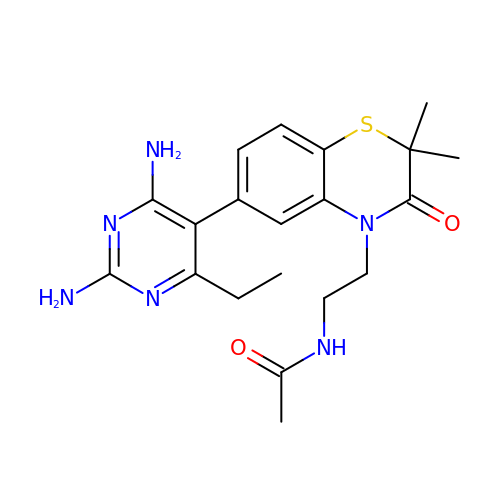N-{2-[6-(2,4-DIAMINO-6-ETHYLPYRIMIDIN-5-YL)-2,2-DIMETHYL-3-OXO-2,3-DIHYDRO-4H-1,4-BENZOTHIAZIN-4-YL]ETHYL}ACETAMIDE | C20 H26 N6 O2 S | RMEVNJZCKDVVND-UHFFFAOYSA-N>GSHMASKVLVLNCGSSSVKYKLLEMPKGDVLAQGGVEKLGLPGSFLKLTMPNGEKVVLEKDMPEHTIAVEFILSVLKDDKYGCIKSYEEIDAVGHRLVHGGEKFSNSVEITPEVIAKVEECIPLAPLHNPANLKGVVAIEKLLPGIRQVGVFDTAFFQTMPEHVYRYALPYDMCNKHGVRRYGFHGTSHRYVSARACEILGLDYDKTRIITAHIGNGASIAAIKNGKALDVSLGMTPVEGLMMGTRSGDVDPGVLTFLMEAEGLQAAGISELINKKSGVLGVSGVSSDLREIEDAIKNGNERATLAMTMYDYRIKKYVGAYAAAMGGVDVLVFTGGVGENQYTTREKVCTDMEFMGIVFDSKVNEGMRGKEMVISKPESKVTVIVVPTDEEYMIASDTMTILK[4x]

Porphyromonas gingivalis, a black-pigmented Gram-negative rod-type bacterium, is a keystone pathogen linked to the onset and progression of periodontitis. In many bacteria, the enzymes phosphotransacetylase (Pta, EC 2.3.1.8) and acetate kinase (Ack, EC 2.7.2.1) form a key pathway for production of ATP from excess acetyl coenzyme A (acetyl-CoA). Pta produces acetyl phosphate (AcP) from acetyl-CoA, and AcP is subsequently converted to acetate by Ack, with the concomitant production of ATP through substrate-level phosphorylation. In the current study, recombinant Pta (PgPta) and Ack (PgAck) from P. gingivalis ATCC 33277, encoded by pta (PGN_1179) and ack (PGN_1178), respectively, were prepared and enzymatically characterized.

The structure of PgAck was refined at 1.9 Å resolution. Four subunits (A, B, C, and D) are present in the asymmetric unit of the P21 cell. Interfaces between subunits A and B, and subunits C and D (interface area of ~3000 Å2) received significantly higher scores than others (data not shown), suggesting that PgAck forms a homodimer, with two homodimers present in the asymmetric unit. The structure of the PgAck subunit is composed of two α/β domains; the N-terminal domain (residues 1–149 and 384–398) and the C-terminal domain (residues 150–383). The C-terminal domain of each subunit is responsible for dimerization, and the dimer is related by the 2-fold symmetry axis. The structure of the C-terminal domain is almost invariant among the subunits, and the positions of the N-terminal domain relative to the C-terminal domain are different, leading to opening and closing of the cleft. The cleft in subunit D is the most closed, with two sulfate ions bound, presumably derived from lithium sulfate in the mother liquor. By contrast, the cleft of subunit D is almost closed in the PgAck structure determined without any ligands such as ADP, AlF3, and acetate. This structure likely represents complete cleft closure because there is a direct contact between residues Glu32 and Arg285 positioned on opposite sides of the interface of the two domains. Arg91 and Arg241 interact with SO42- 401 in the crystal structure, while Glu385 is positioned ~7 Å away from both sulfate ions.> MTDRMTQLQICLDQMTEQFCATLNYIDK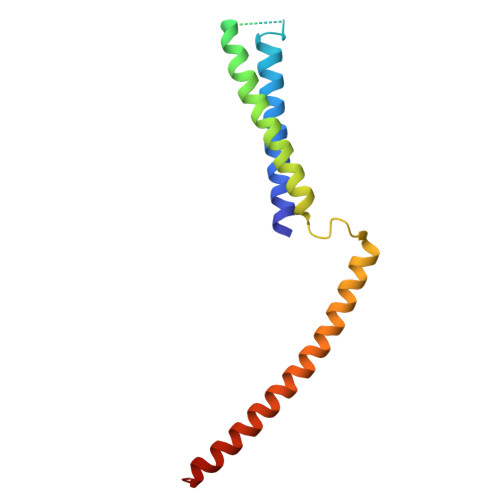NHGFERLTVNEPQMSDKHATVVPPEEFSNTIDELSTDIILKTRQINKLIDSLPGVDVSAEEQLRKIDMLQKKLVEVEDEKIEAIKKKEKLMRHVDSMIEDFVDG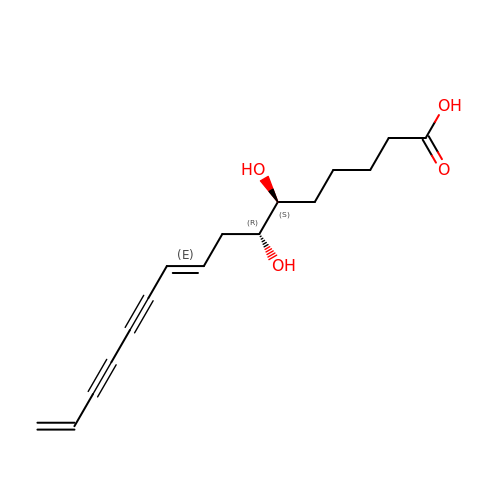(6S,7R,9E)-6,7-bis(oxidanyl)hexadeca-9,15-dien-11,13-diynoic acid | C16 H20 O4 | JBBDMFIFQBMXHD-PEGRTIRESA-N>MAGARRLELGEALALGSGWRHVCHALLYAPDPGMLAGRIPLRYAILMQMRFDGRLGFPGGFVDTQDRSLEDGLNRELREELGEAAAAFRVERTDYRSSHVGSGPRVVAHFYAKRLTLEELLAVEAGATRAKDHGLEVLGLVRVPLYTLRDGVG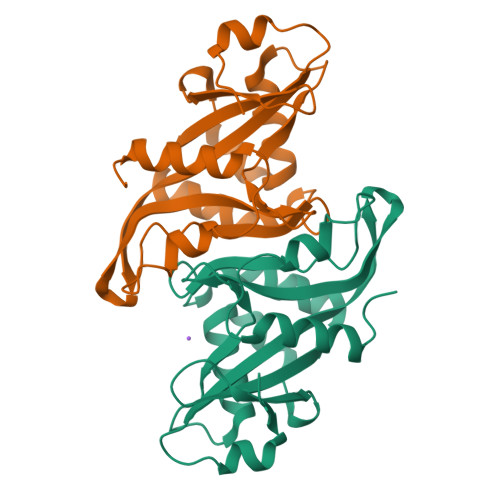GLPTFLENSFIGSAREQLLEALQDLGLLQSGSISGLKIPAHH[2x]>[3x]MKGVIEYSLKTSNDDQFIDITNLVKKAVDESGVSDGMAVVFCPHTTAGITINENADPDVTRDILVNLDKVFPKVGDYKHVEGNSHAHIKASLMGSSQQ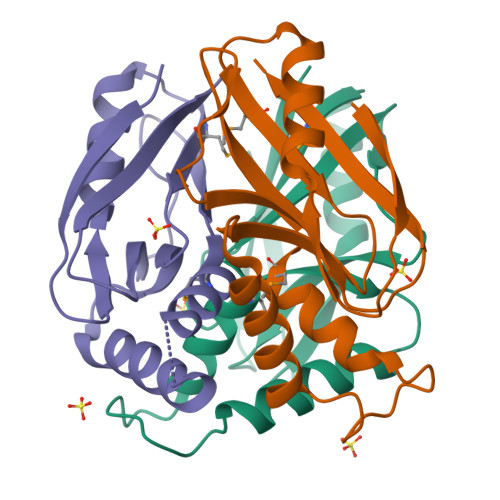IIIENGKLKLGTWQGIYFTEFDGPRDRKVFVKIILEHHHHHH> GSHMNYNPEEQFRCTIIRGKAKNMLDNLLPAYANIIDDICPCDKASFVKDFNNRLIEILGEETTKKTLDNHRTEIAGKLFGMFYEDDEVIFPSGRTNKYIED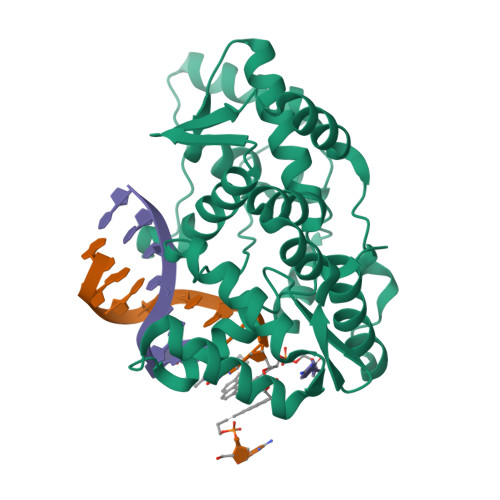SDQPAFFKDICFKFQFPNGMDKLDKVIEKVGAKIQIRQFPYILQVLLTADNNNIQLSKDDIAYYVLNSLQVLQGKIKPIEVIEKIIEDRSNDITKKVRHPGKETSYSMQHIREQLNYLELANLIRIDGNLVKLNYREAENINYIAQFWGNKPEFNAYKYDFTSEDDKKSFFKDWQQYYSNVNSHKS> TLVHVASVEKGRSYEDFQKVYNAIALKLREDDEYDNYIGYGPVLVRLAWHISGTWDKHDNTGGSYGGTYRFKKEFNDPSNAGLQNGFKFLEPIHKEFPWIS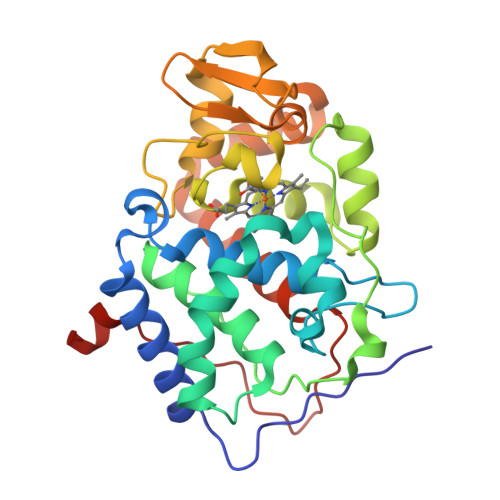SGDLFSLGGVTAVQEMQGPKIPWRCGRVDTPEDTTPDNGRLPDADKDAGYVRTFFQRLNMNDREVVALMGAGALGKTHLKNSGYEGPWGAANNVFTNEFYLNLLNEDWKLEKNDANNEQWDSKSGYMMLPTDYSLIQDPKYLSIVKEYANDQDKFFKDFSKAFEKLLENGITFPKDAPSPFIFKTLEEQGL> STMEELQAA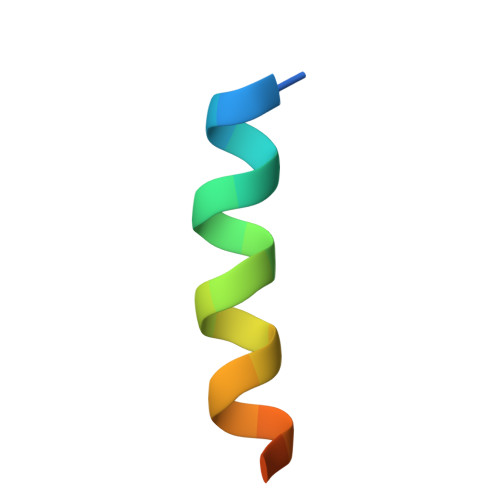IQAAIAHCKNSY> GPLGSETITVPTPIKQIFSDDAFAETIKDNLKKKSVTDAVTQNELNSIDQIIANNSDIKSVQGIQYLPNVTKLFLNGNKLTDIKPLANLKNLGWLFLDENKVKDLSSLKDLKKLKSLSLEHNGISDINGLVHLPQLESLYLGNNKITDIT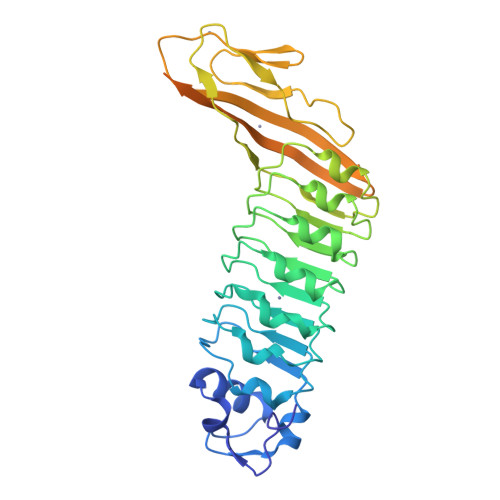VLSRLTKLDTLSLEDNQISDIVPLAGLTKLQNLYLSKNHISDLRALAGLKNLDVLELFSQECLNKPINHQSNLVVPNTVKNTDGSLVTPEIISDDGDYEKPNVKWHLPEFTNEVSFIFYQPVTIGKAKARFHGRVTQPLKEVYTVSYDVDGTVIKTKVEAGTRITAPKPPTKQGYVFKGWYTEKNGGHEWNFNTDYMSGNDFTLYAVFKAET>XGELKAIAQELK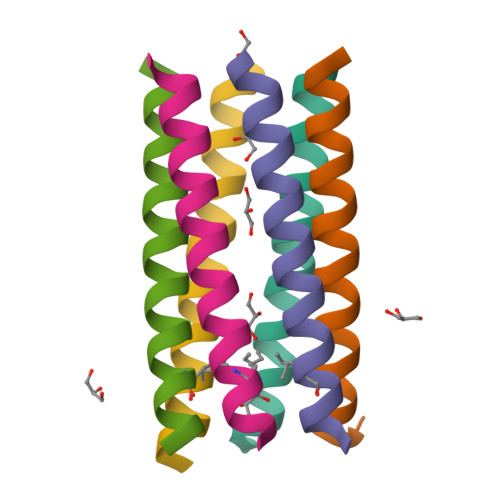AIAKELKAIAWELKAIAQGX[12x]>[8x]MLDFYALEDLLTPEEKEVQKAARRFLEKEALPHIRDWWEEGVFPTHLIPRFAELGFLGPTLPPEYGGAGVSSAAYGLICYELERVDSGLRSFVSVQS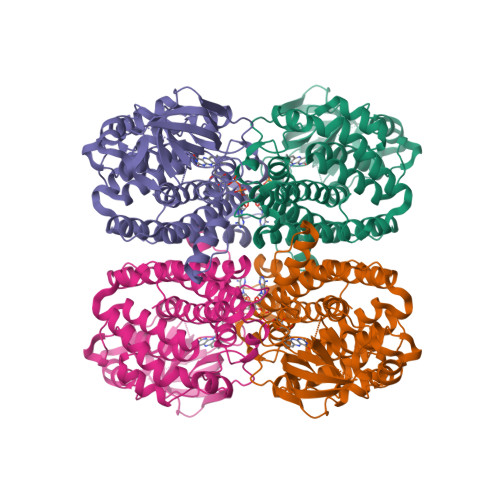SLVMYPIYAYGSEEQKREFLPKLARGEMVGCFGLTEPDGGSDPYGNMKTRARREGDTWVLNGTKMWITNGNLAHLAVIWAKDEGGEVLGFLVPTDTPGFQAREVKRKMSLRASVTSELVLEEVRVPESLRLPKALGLKAPLSCLTQARFGIAWGAMGALEAVYEEAVAFAKSRSTFGEPLAKKQLVQAKLAEMLAWHTEGLLLAWRLARLKDEGKLTPAQVSLAKRQNVWKALQAARMARDILGGSGITLEYHAIRHMLNLETVYTYEGTHDVHTLVLGREITGLNAF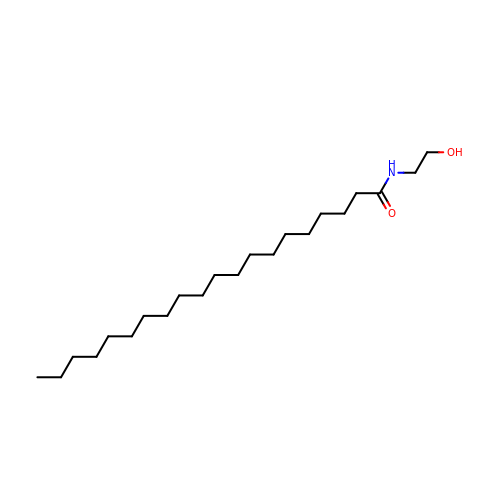N-(2-hydroxyethyl)icosanamide | C22 H45 N O2 | AUJVQJHODMISJP-UHFFFAOYSA-N>[4x]GPGYQDPNNRYSFIGGRTGQWQVVKIRNVLGPGLQLVEKVNILNGAVAEIPLDSAWRLQGFASNIRYAIRTELEALQAVQPMLNRAEAILAVLIPIKKS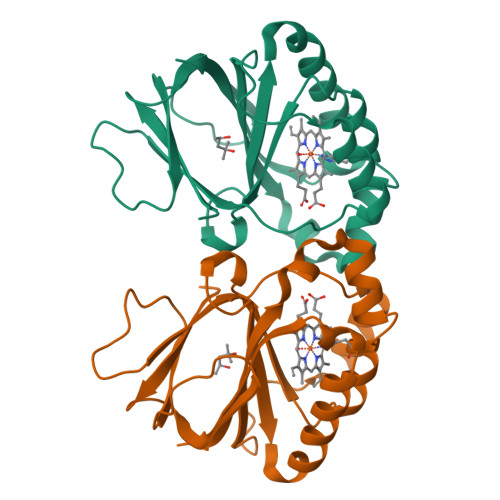AQWWEMAQDERRDIFERESHHTAVGLEYLPGVARRLLHCRDLGEEFDFLTWFEFAPEHSSAFNELLLRMRASKEWEYVEREVEVWLKRL>[4x]MGG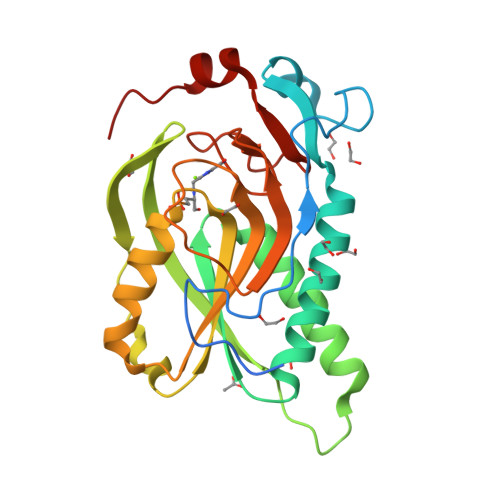SHHHHHHGGLVPRGSHMPIPNNPGAGENAFDPVFVNDDDGYDLDSFMIPAHYKKYLTKVLVPNGVIKNRIEKLAYDIKKVYNNEEFHILCLLKGSRGFFTALLKHLSRIHNYSAVETSKPLFGEHYVRVKSYCNDQSTGTLEIVSEDLSCLKGKHVLIVEDIIDTGKTLVKFCEYLKKFEIKTVAIACLFIKRTPLWNGFKADFVGFSIPDHFVVGYSLDYNEIFRDLDHCCLVNDEGKKKYKATSL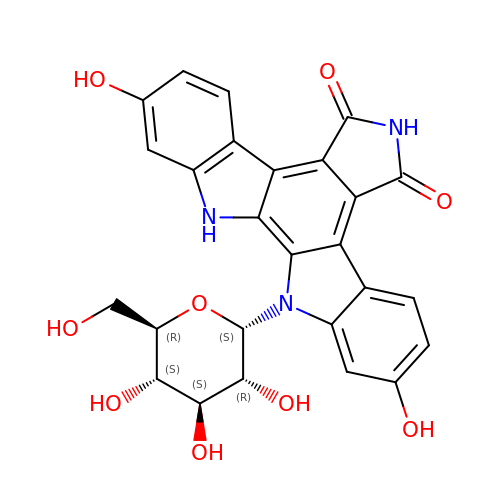2,10-DIHYDROXY-12-(BETA-D-GLUCOPYRANOSYL)-6,7,12,13-TETRAHYDROINDOLO[2,3-A]PYRROLO[3,4-C]CARBAZOLE-5,7-DIONE | C26 H21 N3 O9 | URWNZLQOQBNPOF-FQCBRIBZSA-N>[2x]HHHHHHSSGLVPRGSHMPTPSQHKDASTAQTDNQVPTGRRAQKREQTRARLITSARTLMAER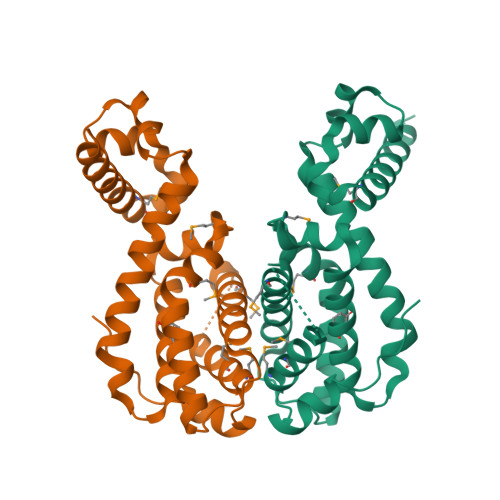GVDNVGIAEITEGANIGTGTFYNYFPDREQLLQAVAEDAFESVGIALDQVLTKLDDPAEVFAGSLRHLVRHSLEDRIWGGFFIQMGAAHPVLMRILGPRARRDLLHGLETGRFTIEDLDLATTCTFGSLIAAIQMALSADQDSNDDKDQIFAAAMLRMVGVQAAEAREIASRPLPEISPVKPQ> GPVLEATMICIDNSEWMRNGDYSPSRLQAQTEAVNLLCGAKTQSNPENTVGILTMAGKGVRVLTTPTSDLGKILACMHGLDVGGEINLTAAIQIAQLALKHRQNKNQRQRIIVFAGSPIKYEKKALEIVGKRLKKNSVSLDIVNFGEDDDEEKPQKLEALLTAVNNNDGSHIVH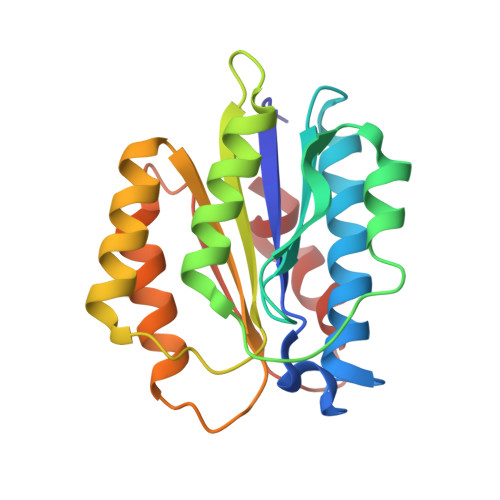VPSGANALSDVLLSTPVFTG> GAMA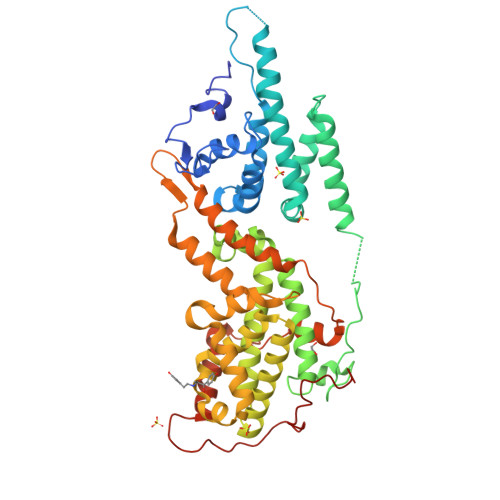EQQLRLPSPEVYRFVVKDSEENIVFEDNLQSRSGIPIIKGGTVVKLIERLTYHMYADPNFVRTFLTTYRSFCKPQELLSLLIERFEIPEPEPTDADKLAIEKGEQPISADLKRFRKEYVQPVQLRILNVFRHWVEHHFYDFERDLYLLERLESFISSVRGKAMKKWVESIAKIIRRKKQAQANGVSHNITFESPPPPIEWHISKPGHIETFDLMTLHPIEIARQLTLLESDLYRKVQPSELVGSVWTKEDKEINSPNLLKMIRHTTNLTLWFEKCIVEAENFEERVAVLSRIIEILQVFQDLNNFNGVLEIVSAVNSVSVYRLDHTFEALQERKRKILDEAVELSQDHFKKYLVKLKSINPPCVPFFGIYLTNILKTEEGNNDFLTRHGKDLINFSKRRKVAEITGEIQQYQNQPYCLRIEPDMRRFFENLNPMGSASEKEFTDYLFNKSLEIEPRNPKQPPRFPRKSTFSLKSPGIRPNTGRHGS>ELNRSQGIPFLEYKHFVTRTFFPKCSSLYEERYVLPSKTLNSQGGSPPQETHPLLGEWNIPEHCRPSMEEGISLFSSLLNNKHFLIVFVHALEQQKDFAVRDRCSLASLLTIALHGKLEYYTSIMKELLVDLIDASAAKNPKLMLRRTESVVEKMLTNWMSICMYGCLRETVGEPFFLLLCAIKQQINKGSIDAITGKARYTLNEEWLLRENIEAKPRNLNVSFQGCGMDSLSVRAMDTDTLTQVKEKILEAFCKNVPYSQWPRAEDVDLEWFASSTQSYVLRDLDDTSVVEDGRKKLNTLAHYKIPEGASLAMSLTDKKDSTLGRVKDLDTEKYFHLVLPTDELVEPKKSHRQSHRKKVLPEIYLTRLLSTKGTLQKFLDDLFKAILSIREDKPPLAVKYFFDFLEEQAEKRGISDPDTLHIWKTNSLPLRFWVNILKNPQFVFDIEKTDHIDACLSVIAQAFIDACSISDLQLGKDSPTNKLLYAKEIPEYRKTVQRYYKQIQDMTPLSEQEMNAHLAEESRKYQNEFNTNVAMAEIYKYAKRYRPQIMAALEANPTARRTQLQHKFEQVVALMENNIYECYSEA[2x]

GIPC1 (GAIP interacting protein, C-terminus 1) and its two paralogs GIPC2 and GIPC3 are universal adaptor proteins that bind and regulate vesicular trafficking of many transmembrane proteins. GIPCs contribute to the endocytosis process by tethering the cargo proteins on endocytic vesicles to the motor protein myosin VI. GIPCs contain a central PDZ (PSD-95, Dlg and ZO-1) domain that mediates the interaction with the C-terminal PDZ-binding motif (PBM) in cargo proteins. The transmembrane receptor PlexinD1 contains a C-terminal ‘SEA’ motif that constitutes a PBM and interacts with GIPC1.

While full-length PlexinD1cyto failed to crystallize, we crystallized and determined the structures of a construct with the JM segment truncated (still referred to as PlexinD1cyto for simplicity), both in the apo-form (to 2.7 Å resolution) and in complex with GIPC1 (to 3.2 Å resolution). The overall structure of apo-PlexinD1cyto are similar to other plexincyto structures reported previously. The RBD forms an independent ubiquitin-like domain that packs against one side of the GAP domain. The two GAP-homology regions (C1 and C2) fold together to form the GAP domain. The GAP domain of plexins contains a regulatory element referred to as the activation segment, which toggles between the closed inactive and open active conformations under the control of plexin dimerization. The activation segment in the PlexinD1cyto structure appears partially open, although it was crystallized in the monomeric state. In the apo-PlexinD1cyto structure, the C-terminal tail region (residues 1916–1925) constitutes the C-terminal part of the last helix in the GAP domain, except for the last two residues (Glu1924 and Ala1925) which are disordered.> SNAIQQSDGSMIIDGSANLRDLNKMFNWELDTEDARTFNGLILEHLEEIPDEG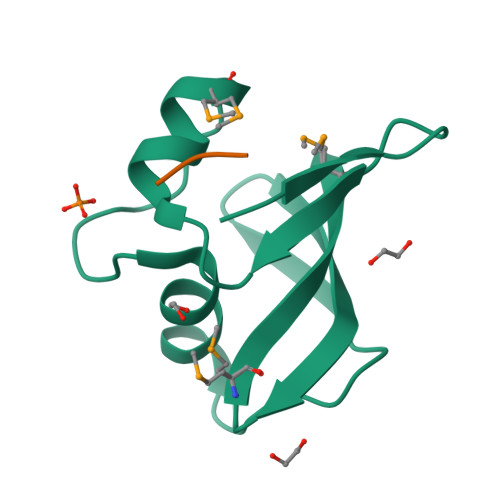TICEIDGLLITILEVGDNMIKQAKVVKL;> IFG>[2x]MGDRGSSRRRRTGSRPSSHGGGGPAAAEEEVRDAAAGPDVGAAGDAPAPAPNKDGDAGVGSGHWELRCHRLQDSLFSSDSGFSNYRGILNWCVVMLILSNARLFLENLIKYGILVDPIQ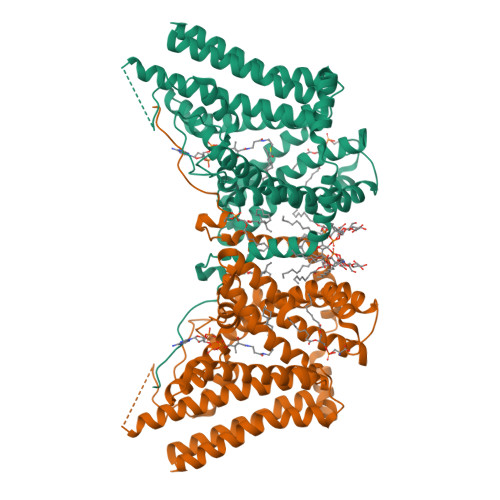VVSLFLKDPYSWPAPCLVIAANVFAVAAFQVEKRLAVGALTEQAGLLLHVANLATILCFPAAVVLLVESITPVGSLLALMAHTILFLKLFSYRDVNSWCRRARAKAASAGKKASSAAAPHTVSYPDNLTYRDLYYFLFAPTLCYELNFPRSPRIRKRFLLRRILEMLFFTQLQVGLIQQWMVPTIQNSMKPFKDMDYSRIIERLLKLAVPNHLIWLIFFYWLFHSCLNAVAELMQFGDREFYRDWWNSESVTYFWQNWNIPVHKWCIRHFYKPMLRRGSSKWMARTGVFLASAFFHEYLVSVPLRMFRLWAFTGMMAQIPLAWFVGRFFQGNYGNAAVWLSLIIGQPIAVLMYVHDYYVLNYEAPAAEA> PPGTVDKKMVEKCWKLMDKVVRLCQNPKLALKNSPPYILDLLPDTYQHLRTILSRYEGKMETLGENEYFRVFMENLMKKTKQTISLFKEGKERMYEENSQPRRNLTKLSLIFSHMLAELKGIFPSGLFQGDTFRITKADAAEFWRKAFGEKTIVPWKSFRQALHEVHPISSGLEAMALKSTIDLTCNDYISVFEFDIFTRLFQPWSSLLRNWNSLAVTHPGYMAFLTYDEVKARLQKFIHKPGSYIFRLSCTRLGQWAIGYVTADGNILQTIPHNKPLFQALIDGFREGFY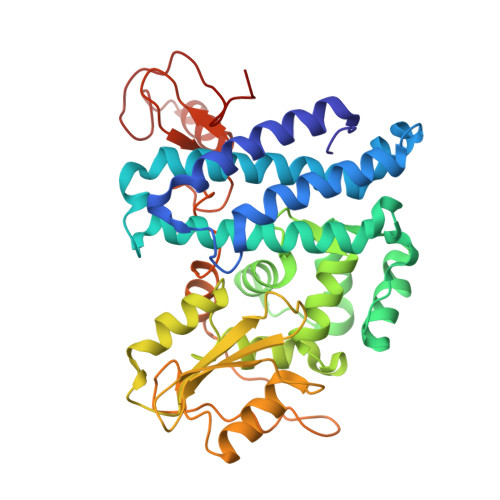LFPDGRNQNPDLTGLCEPTPQDHIKVTQEQYELYCEMGSTFQLCKICAENDKDVKIEPCGHLMCTSCLTSWQESEGQGCPFCRCEIKGTEPIVVDPF>SDKTFLENNQYTDEGVKVYEFIFGENYISSGGLEATKKILSDIELNENSKVLDIGSGLGGGCMYINEKYGAHTHGIDICSNIVNMANERVSGNNKIIFEANDILTKEFPENNFDLIYSRAAILHLSLENKNKLFQKCYKWLKPTGTLLITDYCATEKENWDDEFKEYVKQRKYTLITVEEYADILTACNFKNVVSKDLSDYWNQLLEVEHKYLHENKEEFLKLFS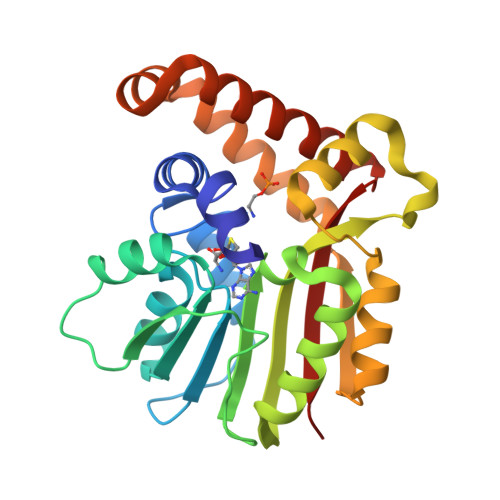EKKFISLDDGWSRKIKDSKRKMQRWGYFKATKN[2x]>GAMGSRLYDRRSIFDAVAQSNCQELESLLPFLQRSKKRLTDSEFKDPETGKTCLLKAMLNLHNGQNDTIALLLDVARKTDSLKQFVNASYTDSYYKGQTALHIAIERRNMTLVTLLVENGADVQAAANGDFFKKTKGRPGFYFGELPLSLAACTNQLAIVKFLLQNSWQPADISARDSVGNTVLHALVEVADNTVDNTKFVTSMYNEILILGAKLHPTLKLEEITNRKGLTPLALAASSGKIGVLAYILQREIHEPECRHLSRKFTEWAYGPVHSSLYDLSCIDTCEKNSVLEVIAYSSSETPNRHDMLLVEPLNRLLQDKWDRFVKRIFYFNFFVYCLYMIIFTAAAYYRPVEGLPPYKLKNTVGDYFRVTGEILSVSGGVYFFFRGIQYFLQRRPSLKSLFVDSYSEILFFVQSLFMLVSVVLYFSQRKEYVASMVFSLAMGWTNMLYYTRGFQQMGIYAVMIEKMILRDLCRFMFVYLVFLFGFSTAVVTLIEDGKYNSLYSTCLELFKFTIGMGDLEFTENYDFKAVFIILLLAYVI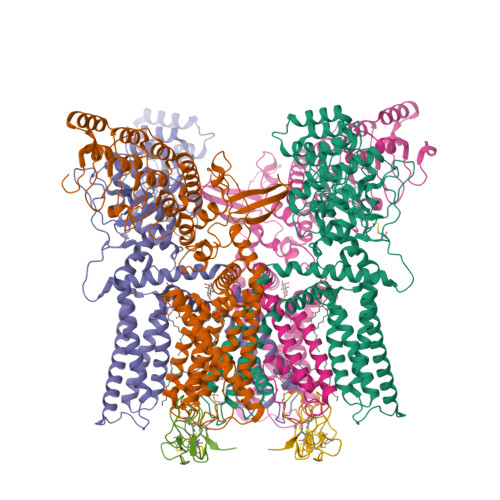LTYILLLNMLIALMGETVNKIAQESKNIWKLQRAITILDTEKSFLKCMRKAFRSGKLLQVGFTPDGKDDYRWCFRVDEVNWTTWNTNVGIINEDPG[4x];>MDCAKEGEVCSWGKKCCDLDNFYCPMEFIPHCKKYKPYVPVTTNCAKEGEVCGWGSKCCHGLDCPLAFIPYCEKYR[2x]>AAPPAPPVSYGVEEDVFHPVRAKQGMVASVDATATQVGVDILKEGGNAVDAAVAVGYALAVTHPQAGNLGGGGFMLIRSKNGNTTAIDFREMAPAKATRDMFLDDQGNPDSKKSLTSHLASGTPGTVAGFSLALDKYGTMPLNKVVQPAFKLARDGFIVNDALADDLKTYGSEVLPNHENSKAIFWKEGEPLKKGDTLVQANLAKSLEMIAENGPDEFYKGTIAEQIAQEMQKNGGLITKEDLAAYKAVERTPISGDYRGYQVYSMPPPSSGGIHIVQILNILENFDMKKYGFGSADAMQIMAEAEKYAYADRSEYLGDPDFVKVPWQALTNKAYAKSIADQIDINKAKPSSEIRPGKLAPYESNQ[2x];>[2x]TTHYSVVDKDGNAVAVTYTLNTTFGTGIVAGESGILLNNQMDDFSAKPGVPNVYGLVGGDANAVGPNKRPLSSMSPTIVVKDGKTWLVTGSPGGSRIITTVLQMVVNSIDYGLNVAEATNAPRFHHQWLPDELRVEKGFSPDTLKLLEAKGQKVALKEAMGSTQSIMVGPDGELYGASDPRSVD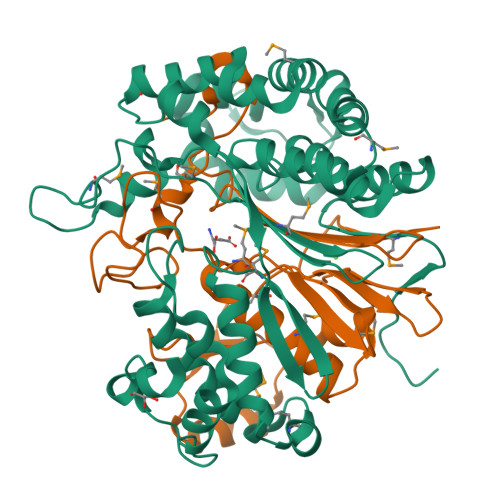DLTAGY> MKHHHHHHHGAAGTSLYKKAGENLYFQGSHLQRNIYLSLLHMEPEEGQEKAPKVPDSVIRAALLRRAVEDIHRIIQIRTAKAACSTLLQRGSVGDDLWQRFLRAEKEMEDELRDVVMEANALVPGWGQIIFQSANEIAANKVLRDRLEEIEAQTARDKE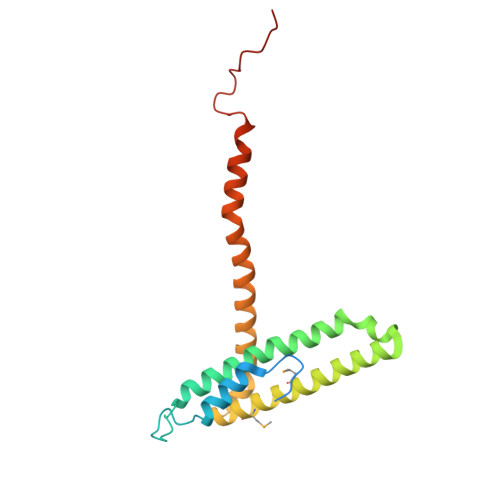WWEKRRATIKSEFMKELDAEEAVEK>[2x]MGSSHHHHHHSQDPNSMLSVGATTTATRLTGWGR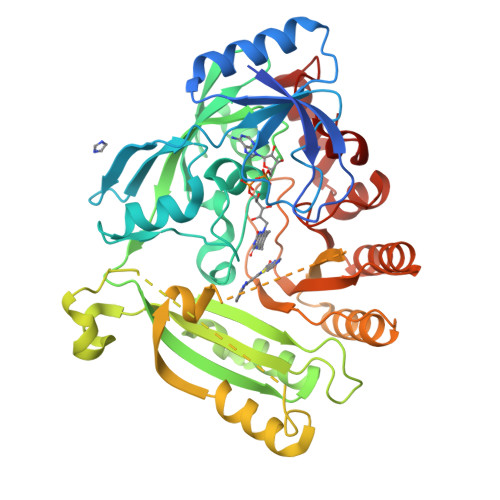TAPSVANVLRTPDAEMIVKAVARVAESGGGRGAIARGLGRSYGDNAQNGGGLVIDMTPLNTIHSIDADTKLVDIDAGVNLDQLMKAALPFGLWVPVLPGTRQVTVGGAIACDIHGKNHHSAGSFGNHVRSMDLLTADGEIRHLTPTGEDAELFWATVGGNGLTGIIMRATIEMTPTSTAYFIADGDVTASLDETIALHSDGSEARYTYSSAWFDAISAPPKLGRAAVSRGRLATVEQLPAKLRSEPLKFDAPQLLTLPDVFPNGLANKYTFGPIGELWYRKSGTYRGKVQNLTQFYHPLDMFGEWNRAYGPAGFLQYQFVIPTEAVDEFKKIIGVIQASGHYSFLNVFKLFGPRNQAPLSFPIPGWNICVDFPIKDGLGKFVSELDRRVLEFGGRLYTAKDSRTTAETFHAMYPRVDEWISVRRKVDPLRVFASDMARRLELL>[2x]MRVGIPTETKNNEFRVAITPAGVAELTRRGHEVLIQAGAGEGSAITDADFKAAGAQLVGTADQVWADADLLLKVKEPIAAEYGRLRHGQILFTFLHLAASRACTDALLDSGTTSIAYETVQTADGALPLLAPMSEVAG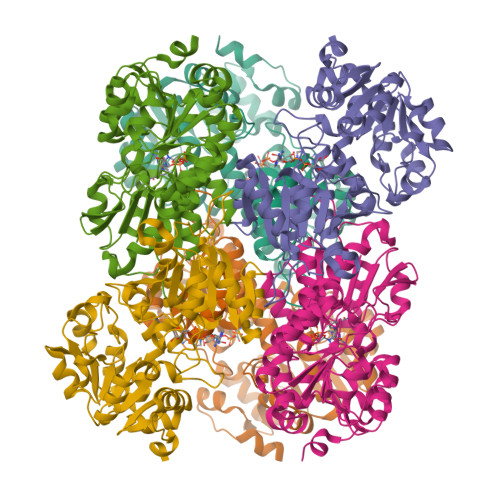RLAAQVGAYHLMRTQGGRGVLMGGVPGVEPADVVVIGAGTAGYNAARIANGMGATVTVLDINIDKLRQLDAEFCGRIHTRYSSAYELEGAVKRADLVIGAVLVPGAKAPKLVSNSLVAHMKPGAVLVDIAIDQGGCFEGSRPTTYDHPTFAVHDTLFYCVANMPASVPKTSTYALTNATMPYVLELADHGWRAACRSNPALAKGLSTHEGALLSERVATDLGVPFTEPASVLAHHHHHH>MGSSHHHHHHENLYFQGSMEQAIINDEREYLRHFWHPVCTVTELEKAHPSSLGPLAVKLLNEQLVVAKLGDEYVAMRDRCAHRSAKLSLGTVSGNRLQCPYHGWQYDTHGACQLVPACPNSPIPNKAKVDRFDCEERYGLIWIRLDSSFDCTEIPYFSAANDPRLRIVIQEPYWWDATAERRWENFTDFSHFAFIHPGTLFDPNNAEPPIVPMDRFNGQFRFVYDTPEDMAVPNQAPIGSFSYTCSMPFAINLEVSKYSSSSLHVLFNVSCPV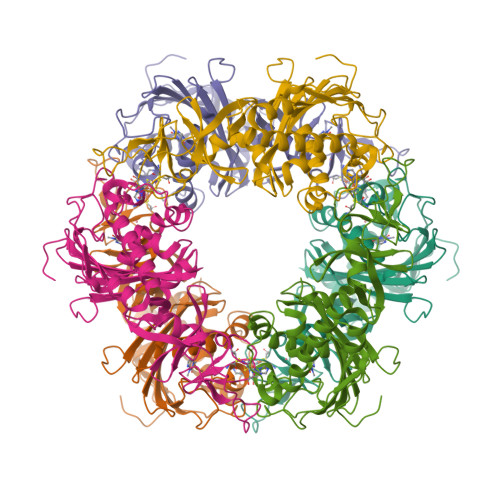DSHTTKNFLIFAREQSDDSDYLHIAFNDLVFAEDKPVIESQWPKDAPADEVSVVADKVSIQYRKWLRELKEAHKEGSQAFRSALLDPVIESDRSYI[3x]> MHKEAHFTAGEIVRDIIIGVSDGLTVPFALAAGLSGANASSSI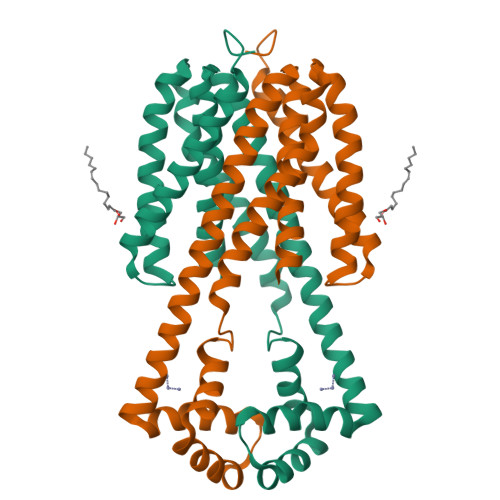VLTAGIAEVAAGAISMGLGGYLAAKSEADNYARELKREQEEIIRVPDTEAAEVAEILARYGIEPHEYGPVVNALRKKPQAWLDFMMKFELGLEKPDPKRALQSAFTIAIAYVLGGLVPLIPYMFIPVARKAVVASVILTLMALLIFGYAKGYFTDNKPFKSALQTALIGAIASAAAFGMAKAVQSENLYFQ> MTERSVVHSTFIIERLYPAPPSKVFFALGNADAKRRWFTDPDNPMPGRFEMDFRVGGKEVNAGGPKDGPIHVYTATYQDIVPDQRIVYSYDMLFGETRISVSLATIQLFAEGEGTRLVLTEQGAFLDGHDTPSTREHGTGVLLDLLDAFLD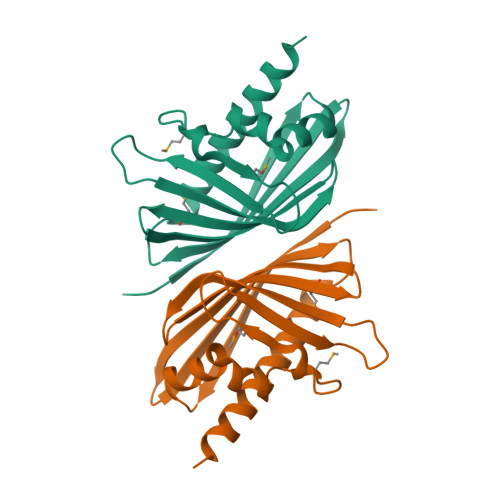KTTLEHHHHHH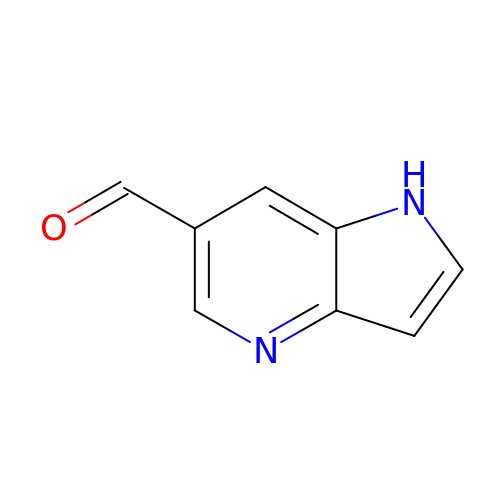1H-pyrrolo[3,2-b]pyridine-6-carbaldehyde | C8 H6 N2 O | HRLUESWIQOAEBQ-UHFFFAOYSA-N Betulinic acid | C30 H48 O3 | 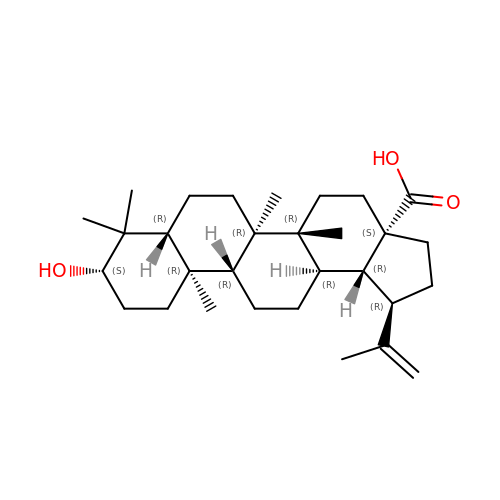QGJZLNKBHJESQX-FZFNOLFKSA-N>GPKSSDHVDLPYNLTATKIDSDVFVVTDRDFYSSNVLVAKMLDGTVVIVSSPFENLGTQTLMDWVAKTMKPKKVVAINTHFHLDGTGGNEIYKKMGAETWSSDLTKQLRLEENKKDRIKAAEFYKNEDLKRRILSSHPVPADNVFDLKQGKVFSFSNELVEVSFPGPAHSPDNVVVYFPKKKLLFGGCMIKPKELGYLGDANVKAWPDSARRLKKFDAKIVIPGHGEWGGPEMVNKTIKVAEKAVGEMRL[2x]

The São Paulo MBL (SPM‐1) is widely distributed in South America, Europe and North America, in the Gram‐negative pathogen Pseudomonas aeruginosa. Like other B1 MBLs (NDM, VIM and IMP),10 SPM‐1 has a binuclear zinc center, but has loop characteristics of the B2 MBLs, suggesting it is a B1/B2 hybrid, which, consequently, may be challenging to inhibit. SPM‐1, like other B1 MBLs, has a di‐zinc ion active site with one zinc ion bound at a (normally tetrahedral) tri‐histidine site (Zn1) and one in a trigonal bipyramidal site (Zn2) comprised of conserved Asp, Cys, and His residues. SPM‐1 is distinguished from other B1 MBLs in possessing a “wall” of hydrophobic residues involving Phe57 and Tyr58 on its L3 loop, Phe79 on the loop connecting α5 and α1, and Phe151 and Tyr152 on the kinked α3 helix in the “closed” form, as well as Tyr228 on the opposite side of the active site cleft.

We then worked to obtain a structure of cyclobutanone 1 complexed to SPM‐1 by soaking crystals with excess inhibitor. The resolution extended to 1.7 Å for uncomplexed crystals and 2.38 Å for inhibitor soaked crystals. Electron density maps for the latter indicated clear Fo‐Fc difference density in the active site into which 1 was modelled as its hydrated form. Wat1 “bridges” the zinc ions and is proposed to act as the “catalytic” nucleophile.10a Relative to uncomplexed SPM‐1 in the same crystal form, a small (∼0.5 Å) movement of Zn2 into a more solvent‐exposed position in the active site is observed; however, the binding of 1 does not cause significant structural effects on the metal center with little change in Zn–Wat1; Zn1–Zn2 or Zn:protein ligand distances. Notable interactions made by 1 are in the vicinity of Zn2. The C4 carboxylate of 1 makes direct interactions with both Zn2 (2.48 Å distance) and Lys219 (2.91 Å), a binding mode likely involved in substrate carboxylate binding in most B1 MBLs. By contrast, 1 makes only weak interactions with Zn1, with the two oxygen atoms of the C6 ketone hydrate with Zn1‐oxygen distances of 3.5 and 4.0 Å. In contrast to previous predictions about cyclobutanone binding to MBLs,14 the Zn‐bridging Wat1 is clearly present, potentially interacting with both the C6 oxygens of 1 (2.7 Å). Binding of 1 involves hydrophobic interactions with several of these, notably involving sandwiching of the bicyclic ring of 1 between the aromatic rings of Tyr58 (consistent with the 19F‐NMR results) and Tyr228, and edge‐face interactions of 1 with Phe79. The Tyr152 side chain is more distant from 1, with its OH group 6.5 (chain A) or 10.8 Å (chain B) away from the C7 atom of 1, again consistent with the 19F NMR results.>MSSKPKPIEIIGAPFSKGQPRGGVEKGPAALRKAGLVEKLKETEYNVRDHGDLAFVDVPNDSPFQIVKNPRSVGKANEQLAAVVAETQKNGTISVVLGGDHSMAIGSISGHARVHPDLCVIWVDAHTDINTPLTTSSGNLHGQPVAFLLKELKGKFPDVPGFSWVTPCISAKDIVYIGLRDVDPGEHYIIKTLGIKYFSMTEVDKLGIGKVMEETFSYLLGRKKRPIHLSFDVDGLDPVFTPATGTPVVGGLSYREGLYITEEIY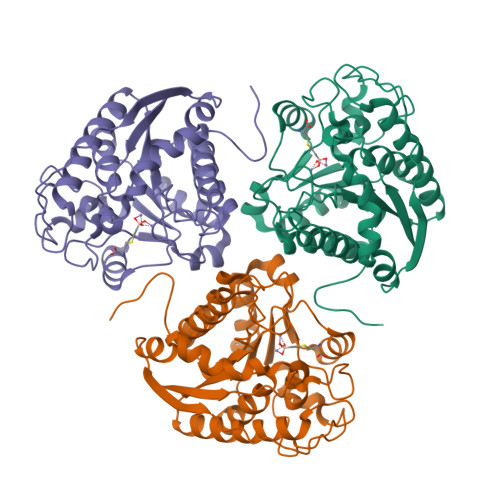KTGLLSGLDIMEVNPTLGKTPEEVTRTVNTAVALTLSCFGTKREGNHKPETDYLKPPK[2x]>GTGAMKDGMRVGERFTHDFVVPPHKTVRHLYPESPEFAEFPEVFATGFMVGLMEWACVRAMAPYLEPGEGSLGTAICVTHTAATPPGLTVTVTAELRSVEGRRLSWRVS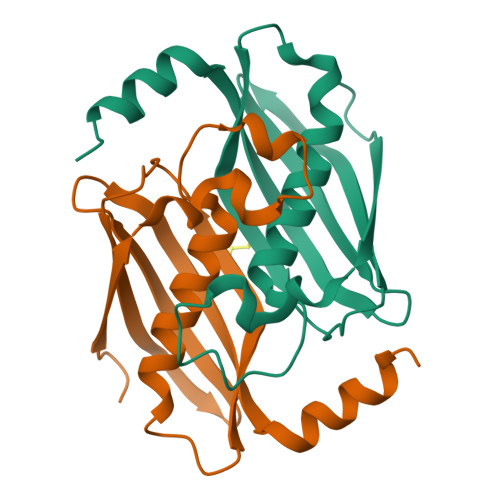AHDGVDEIGSGTHERAVIHLEKFNAKVRQKTPAG[2x]> GPAAASTKVLYYTDRSLTPFLVNIPKRLGDVTLQDFKAAVDRHGSFRYHFKSLDPEFGTVKEEVFQDDAVIPGWEGKIVAWVEED

Three proteins, Dvl, Ccd1, and Axin, play an important role in β-catenin-mediated transcription through formation of a transient molecular complex which is translocated to the plasma membrane in the canonical Wnt pathway. Furthermore, Dvl, Ccd1, and Axin can directly interact with each other through their DIX domains which form the same head-to-tail structures. The mCcd1 and zCcd1 DIX domains have a ubiquitin-like fold with five β-strands and one short α-helix. DIX domains of mCcd1 and zCcd1 are arranged into head-to-tail helical filaments by parallel β-bridge interactions.

In contrast, the zCcd DIX domain is assembled into single-helical filament-like structures consisting of six or seven molecules per turn with a pitch of ~80 Å. The mCcd1 DIX domain was mainly eluted as a monomer with a molecular mass of 10 kDa, whereas the zCcd1 DIX domain was eluted as a dimer with an apparent molecular mass of 19.0 kDa with its monomer included as a minor state in the elution peak. Consistent with this, the accessible surface area in the homomeric head-to-tail interface of the zCcd1 dimer is 590.7 Å2. In addition, the interface of the zCcd1 dimer has two water-mediated hydrogen bonds. In Site 2 of zCcd1, Glu436 (strand β5) in the head-binding molecule have two characteristic electrostatic interactions with Arg368 and Arg395; however, no interaction is observed at the same position in the mCcd1 dimer. Moreover, the side chain of His402 (strand β3) in the head-binding molecule forms hydrogen bonds with Tyr364 via two water molecules. These results suggest that unique interactions observed in zCcd1 may contribute to stabilization of the single-helical polymer. On the other hand, Site 2 interface in zCcd1 was stabilized by two electrostatic interactions of Glu436 with Arg368 and Arg395 in the single-helical filament, despite residue conservation in loop β1-β2 of mCcd1. Phe397 of mCcd1, which is close to the contact surface with loop β1-β2, is replaced with Tyr365 in zCcd1, thereby changing the molecular surface from hydrophobic in mCcd1 to negatively charged in zCcd1. The substitution of Tyr365 with Phe in zCcd1 DIX decreased the apparent molecular weight of the mutant compared to the wild type molecule, making it comparable with that of mCcd1 DIX.> MSNDEKEKLKELLKRAEELAKSPDPEDLKEAVRLAEEVVRERPGSNLAKKALEIILRAAEELAKLPDPEALKEAVKAAEKVVREQPGSNLAKKALEIILRAAEELAKLPDPEALKEAVKAAEKVVREQPG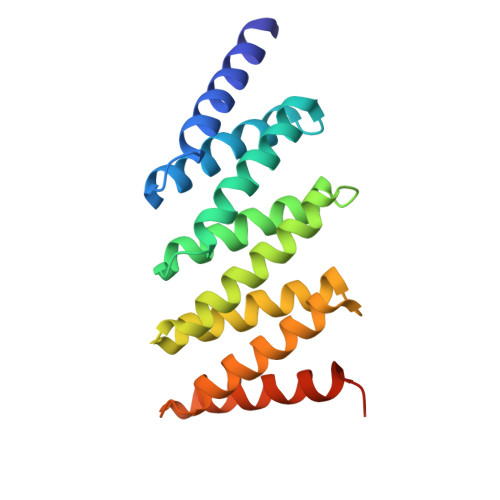SELAKKALEIIERAAEELKKSPDPEAQKEAKKAEQKVREERPGGWLEHHHHHH> MPGLSC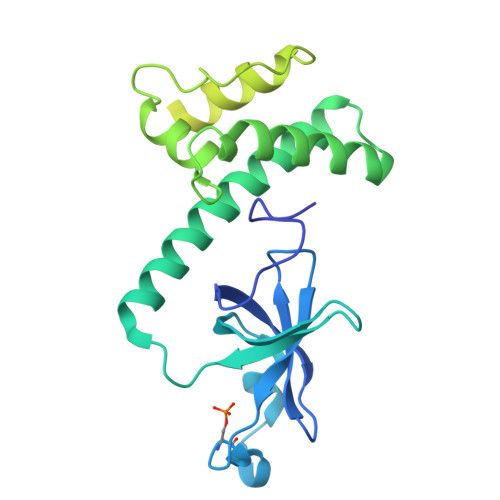RFYQHKFPEVEDVVMVNVRSIAEMGAYVSLLEYNNIEGMILLSELSRRRIRSINKLIRIGRNECVVVIRVDKEKGYIDLSKRRVSPEEAIKCEDKFTKSKTVYSILRHVAEVLEYTKDEQLESLFQRTAWVFDDKYKRPGYGAYDAFKHAVSDPSILDSLDLNEDEREVLINNINRRLTPQAVKIRADIEVACYGYEGIDAVKEALRAGLNCSTENMPIKINLIAPPRYVMTTTTLERTEGLSVLSQAMAVIKEKIEEKRGVFNVQMEPKVVTDTDETELARQMERLERENAEVDGDDDAEEMEAKAED>VDFLPPVGVENREPADATIREKRAKIKEMMTHAWNNYKRYAWGLNELKPISKEGHSSSLFGNIKGATIVDALDTLFIMGMKTEFQEAKSWIKKYLDFNVNAEVSVFEVNIRFVGGLLSAYYLSGEEIFRKKAVELGVKLLPAFHTPSGIPWALLNMKSGIGRNWPWASGGSSILAEFGTLHLEFMHLSHLSGDPVFAEKVMKIRTVLNKLDKPEGLYPNYLNPSSGQWGQHHVSVGGLGDSFYEYLLKAWLMSDKTDLEAKKMYFD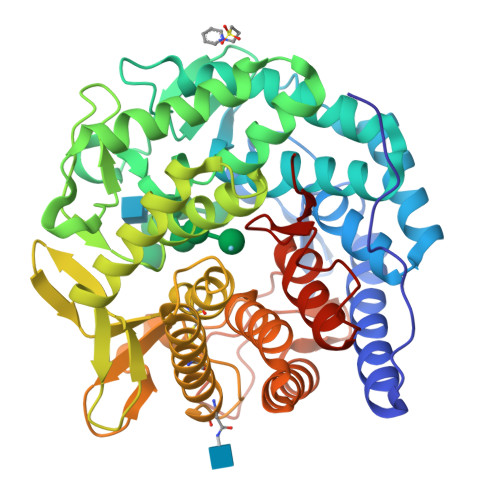AVQAIETHLIRKSSGGLTYIAEWKGGLLEHKMGHLTCFAGGMFALGADGAPEARAQHYLELGAEIARTCHESYNRTYVKLGPEAFRFDGGVEAIATRQNEKYYILRPEVIETYMYMWRLTHDPKYRTWAWEAVEALESHCRVNGGYSGLRDVYIARESYDDVQQSFFLAETLKYLYLIFSDDDLLPLEHWIFNTEAHPFPILR[2x]(2S)-3-[(4-cyanonaphthalen-1-yl)oxy]-N-[4-cyano-3-(trifluoromethyl)phenyl]-2-hydroxy-2-methylpropanamide | 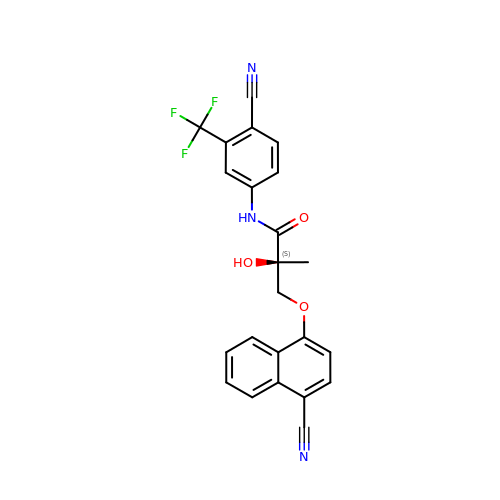C23 H16 F3 N3 O3 | BCJNRNBOQWJRIM-QFIPXVFZSA-N> EAEAYVEFDSFWFVQQWPPAVCSFQKSGSCPGSGLRTFTIHGLWPQQSGTSLTNCPGSPFDITKISHLQSQLNTLWPNVLRANNQQFWSHEWTKHGTCSESTFNQAAAFKLAVDMRNNYDIIGALRPHAAGPNGRTKSRQAIKGFLKAKFGKFPGLRCRTDPQTKVSYLVEVVACFAQDGSTLIDC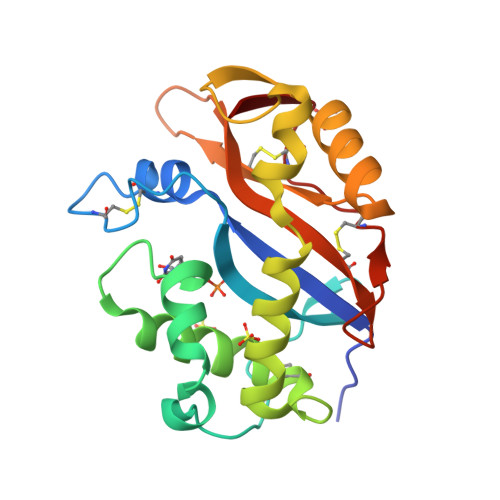TRDTCGANFIF The T6SS of Pseudomonas aeruginosa is a complex machine that the bacterium uses to intoxicate neighboring cells. Among the toxins this system delivers is type VI secretion exported 2 (Tse2). In addition to acting on competing organisms, this toxin can act on P. aeruginosa; thus, the organism synthesizes a protein, type VI secretion immunity 2 (Tsi2), which neutralizes the toxin. Our structure of Tsi2 shows that the protein adopts a dimeric configuration; however, we find that its dimerization is not required for Tse2 interaction.

To gain additional mechanistic insights into Tsi2 function, we solved its X-ray crystal structure to a resolution of 1.00 Å. A molecular model fit to a 1.68 Å resolution electron density map was used to calculate phases for a 1.00 Å data set collected from an isomorphous crystal of native Tsi2–H6. Two monomers interacting through extensive contacts were modeled into the crystallographic asymmetric unit. In the observed Tsi2 dimer, the long axes of the two monomers are arranged approximately perpendicular to each other and the molecules pack via their coiled-coils. This interaction involves a large (725 Å2, 13% total surface area) and predominately hydrophobic (68%) surface area, indicative of a physiologically relevant interface. In agreement with this, the molecular weight of purified Tsi2 measured by gel filtration chromatography was found to closely approximate that of the dimer (calculated, 19.16 kDa; measured, 19.46 kDa), and we observed strong interaction between Tsi2 monomers using the B2H assay. Superimposition of the Tsi2 monomers showed that overall the two subunits adopt highly similar structures (Cα r.m.s.d, 1.1 Å). Interestingly, modeling of the electrostatic surface potential of Tsi2 showed that residues in the vicinity of Glu38, including Asp23, Asp45 and Asp49, generate a prominent negatively charged surface feature. From these data, we conclude that Glu38 and Asp45 of Tsi2 are major determinants of Tse2 interaction. Taken together with our screening data, we conclude that the regions of Tsi2 important for Tsi2 homotypic versus Tse2 heterotypic interactions are topologically distinct; Tse2 binding occurs at the face of Tsi2 opposite the site of homodimerization.

>[2x]MNLKPQTLMVAIQCVAARTRELDAQLQNDDPQNAAELEQLLVGYDLAADDLKNAYEQALGQYSGLPPYDRLIEEPASLEHHHHHH> MECYRCGVSGCHLKITCSAEETFCYKWLNK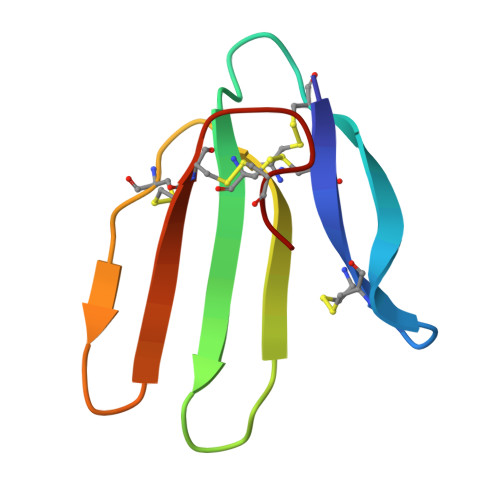ISNERWLGCAKTCTEIDTWNVYNKCCTTNLCNT> GLPGSMNDRADFVVPDITTRKNVGLSHDANDFTLPQPLDRYSAEDHATWATLYQRQCKLLPGRACDEFLEGLERLEVDADRVPDFNKLNEKLMAATGWKIVAVPGLIPDDVFFEHLANRRFPVTWWLREPHQLDYLQEPDVFHDLFGHVPLLINPVFADYLEAYGKGGVKAKALGALPMLARLYWYTVEFG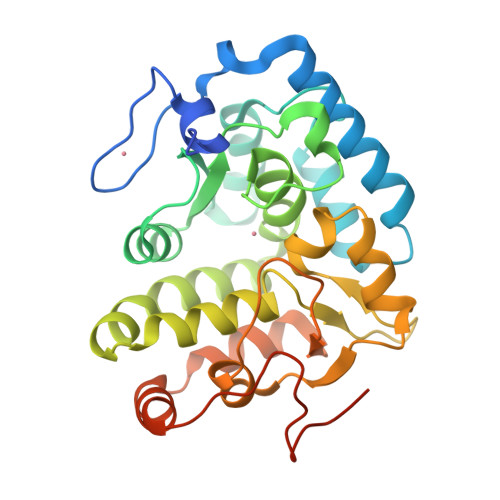LINTPAGMRIYGAGILSSKSESIYCLDSASPNRVGFDLMRIMNTRYRIDTFQKTYFVIDSFKQLFDATAPDAAPLYLQLADAQPWGAGDIAPDDLVLNAGDHQGWADTEDV>[5x]PSESADPHELNEPRILTTDREAVAVAFSPGGSLLAGGSGDKLIHVWDVASGDELHTLEGHTDWVRAVAFSPDGALLASGSDDATVRLWDVAAAEERAVFEGHTHYVLDIAFSPDGSMVASGSRDGTARLWNVATGTEHAVLKGHTDYVYAVAFSPDGSMVASGSRDGTIRLWDVATGKERDVLQAPAENVVSLAFSPDGSMLVHGSDSTVHLWDVASGEALHTFEGHTDWVRAVAFSPDGALLASGSDDRTIRLWDVAAQEEHTTLEGHTEPVHSVAFHPEGTTLASASEDGTIRIWPIATE

The tPkwA was the first prokaryotic WD40 protein isolated from the Thermomonospora curvata, which is a thermophilic actinomycete isolated from composted stable manure. In this work, we expressed and purified the WD40 domain of tPkwA (referred as tPkwA-C), and performed a systematic study on its stability, thermodynamics and folding kinetics. In summary, our current studies showed that tPkwA-C, a prokaryotic protein is a WD40 domain with reversible unfolding property and thermo-stability. Structural analysis and biophysical characterization reveal tPkwA-C is a typical WD40 protein with extraordinary thermodynamic properties.

The three-dimensional structure of tPkwA-C was determined by molecular replacement with the model from our WDSP server and was refined to a resolution of 2.6 Å. The solved structure in P1 space group has five molecules in one asymmetric unit. Each molecule of tPkwA-C in the ASU folds into a seven-bladed β propeller with amino acid residues 449–738. The blades 1–7 were arranged around a pseudo seven-fold axis in sequential order and generated a water accessible channel in the middle of the propeller. Structure alignment of the five molecules showed that Chain B had the most significant conformational change from the other ones, and the most variable regions are among strand Ds and loops on top and bottom surfaces, which are supposed to be the interfaces for interacting with other proteins. More specific structural features contributing to stability are further revealed by crystal structure of tPkwA-C. The hydrophobic cores in the lower part of tPkwA-C surrounding the Phe 467 and Trp 485 seemed to be major factors stabilizing the structure. From the comparison of five molecules in ASU, we can see that these residues are buried inside the tPkwA-C structure, and exhibited little conformational variation between different molecules in ASU. Unlike other Tryptophans of WD doublets, Trp486 and Trp 653 do not form any hydrogen bond with other amino acid residues. In the crystal of tPkwA-C, they adopted two different conformations and caused the conformational variations in the surrounding region. Compared to the Trp486 in chain C, the Trp486 of chain B flipped its indole ring, with quite significant conformational change of the surrounding residues.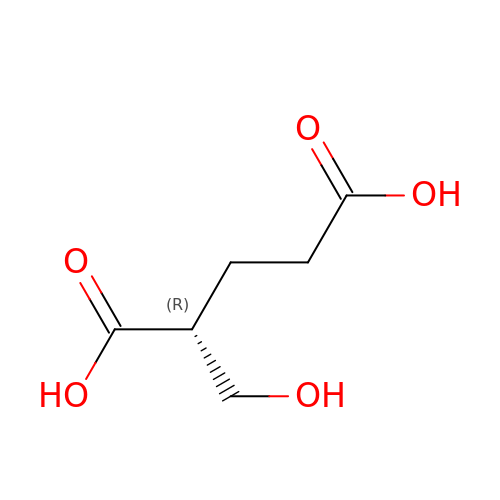(2R)-2-(hydroxymethyl)pentanedioic acid | C6 H10 O5 | XPQIPNORJZZYPV-SCSAIBSYSA-N>[2x]VDKRESYTKEDLLASGRGELFGAKGPQLPAPNMLMMDRV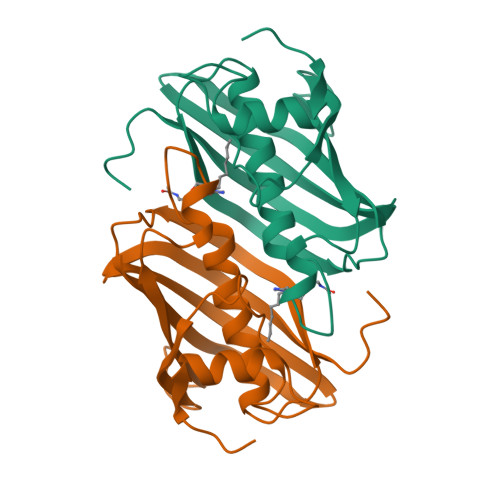VKMTETGGNFDKGYVEAELDINPDLWFFGCHFIGDPVMPGCLGLDAMWQLVGFYLGWLGGEGKGRALGVGEVKFTGQVLPTAKKVTYRIHFKRIVNRRLIMGLADGEVLVDGRLIYTASDLKVGLFQDTSAF>GSPGISGGGGGSPYADSFKEFTNIDEARAWGDKQFAKYKLSSSEKNALTIYTRNAARINGPLRANQGNTNGLPADIRKEVEQIDKSFTKMQTPENIILFRGDDPGYLGPDFENTILNRDGTINKAVFEQVKLRFKGKDRKEYGYISTSLVNGSAFAGRPIITKFKVLDGSKAGYIEPISTFKGQLEVLLPR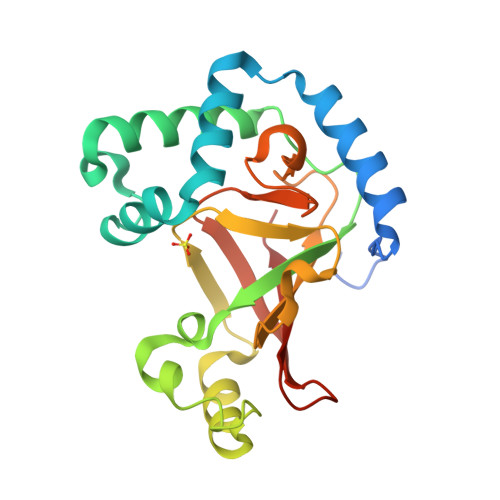SSTYTISDMQIAPNNKQIIITALLKR[2x]>MSLFNVASLKYKHHESIQMIIDRIDHLVLTVSDISTTIRFYEEVLGFSAVTFKQNRKALIFGAQKINLHQQEMEFEPKASRPTPGSADLCFITSTPINDVVSEILQAGISIVEGPVERTGATGEIMSIYIRDPDGNLIE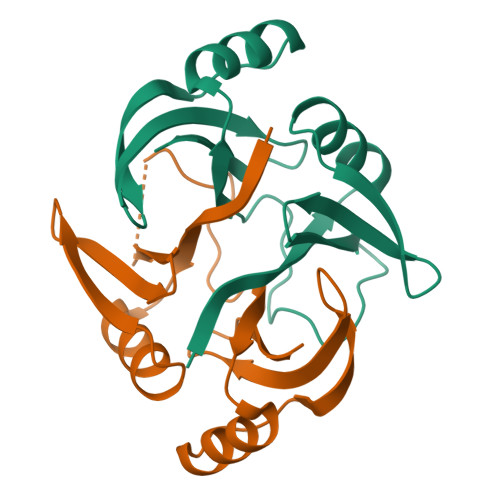ISQYVEGHHHHHH[4x]O-phosphono-N-(8-sulfanyloctanoyl)-L-threonine 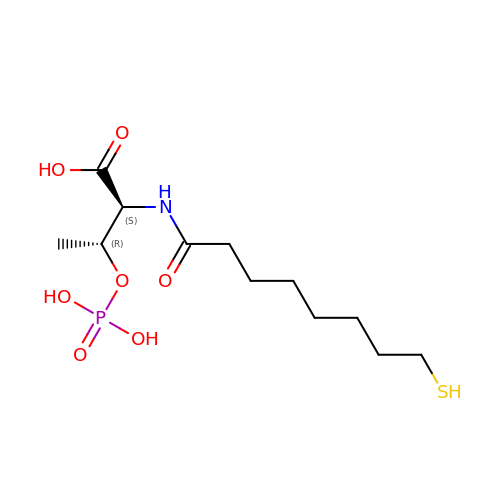| C12 H24 N O7 P S | WKMFNKCCBNAWBN-KOLCDFICSA-N>MAMTVTEVDLPPIYCPLESAIHPRVHEVEKRAVEWIRRSGMCASEEERAWVIATHSADFFARFAPTAADEDRLLATSLWVYWGFAFDDHRCDNGPLSTRPAQFNALAGRVQRALEAPSAEDNGDRFVPALQDIARRFRSFGTPTQVRRFVHAHRA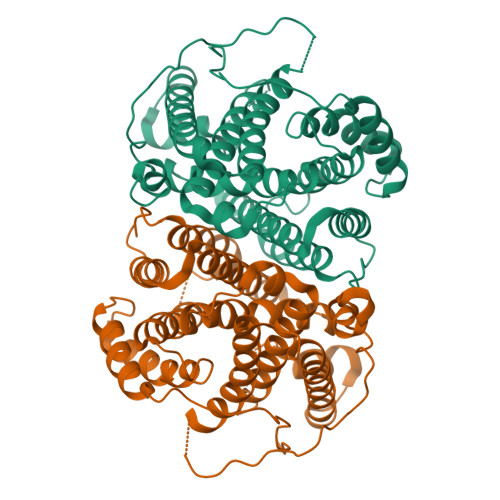WLSGVAWQIGNQARGHMPGLDDYLAMRLLSAGGEPTFAMLEIATGAEVPDREMHRPAVRALTEMAIMVIALDNDRHSLRKELSRGHTDQNIYSVLMHHRGMSLQEAVEEATKLRDRILLRFLELHDRVRPGAGAELSTYLQGLRHGIRGNAEWGLRVPRYLSLGRVPDPMEDAPLTWAESPSDSSPSPLPGAPSIAWWWDDALLGA[2x]> MDPGTVLEISRSLKKRMQ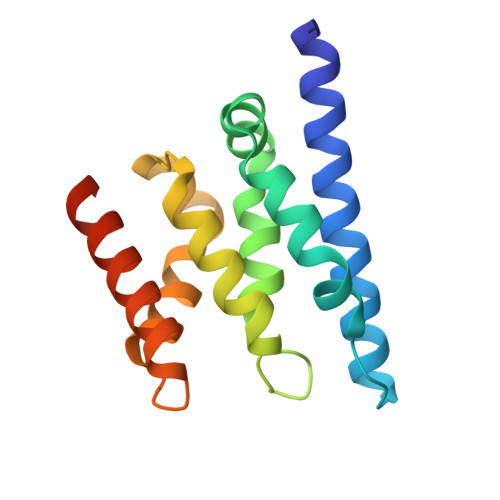DILKKDNANNLEGRPATGKIENVEEISDILMSKALQESLLDEGILDEIKGWLEPLPDKSMPNIKIRKRLLDVLKTMKIHKEHLVTSGVGKIVYFYSINPKESKEVRASAKALVQKWTNEVFKPEGGD>[2x]GMTSPVAVIARFMPRPDARSALRALLDAMITP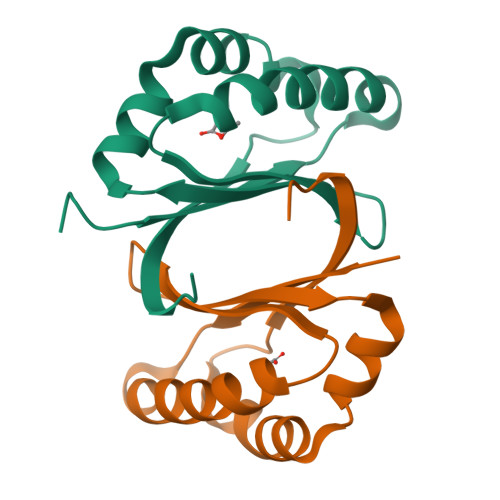TRAEDGCRSYDLYESADGGELVLFERYRSRIALDEHRGSPHYLNYRAQVGELLTRPVAVTVLAPLDEASA ethyl (4S)-5-[(3S)-2-oxopyrrolidin-3-yl]-4-[(3-phenylpropanoyl)amino]pent-2-enoate | 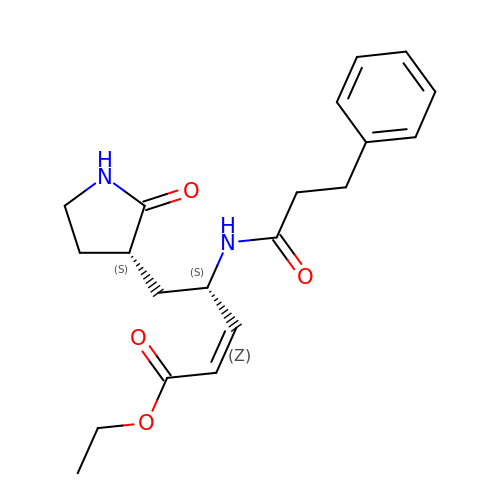C20 H26 N2 O4 | QZQFSCIYJVNTSL-UMYABFQBSA-N The potassium ion efflux channel GORK plays a critical role in closing plant leaf stomata by releasing K+ from guard cells to reduce guard cell volume and turgor. The GUARD CELL OUTWARD-RECTIFYING K+ (GORK) channel is expressed in Arabidopsis guard cells and encodes a K+out channel. Voltage-dependent K+ channels, including GORK, contain three regions: an intracellular N-terminal region, a transmembrane region, and an intracellular C-terminal region (27–30). The transmembrane region is composed of six transmembrane helices (S1-S6), with S1-S4 forming the voltage sensing domain and S5 and S6 forming the pore region.

As a result, five different structures of GORK ranging from the transmembrane region to the C-terminal ANK (designated as GORKWT1–GORKWT5) were determined at resolutions of 3.16 to 3.27 Å. The five GORK structures showed N-terminally an almost uniform transmembrane domain (positions 50 to 313 from the initial Met), including the voltage-sensing domain and the ion selectivity filter. In contrast, the following cytosolic regions, i.e., C-linker (positions 314 to 364), CNBD (positions 365 to 490), CNBD–Ankyrin bridge (positions 491 to 542), and ANK (positions 543 to 722) show five distinct structures in almost twofold symmetry (C2 symmetry). Furthermore, overlaying GORKWT1 and GORKWT5, which had high resolutions of 3.17 and 3.16 Å, respectively, revealed that one of the C-linkers in each dimer was pushed upward by the CNBD in GORKWT1, as compared to GORKWT5. Closer inspection of the structure revealed that the difference of the degree of bending in the C-linker between Mol I and Mol II was small in GORKWT1 but greater in GORKWT5. Additionally, GORKWT1 displayed a C4-like C2 symmetry in the CNBD, whereas GORKWT5 showed a pronounced C2 symmetry. Furthermore, we found a structural difference in the short structure that lies between the CNBD and ANK domains, termed as CNBD–Ankyrin bridge containing residues 511 to 519. This region had an α-helical structure in GORKWT1, while in GORKWT5, it was entirely present in a nonhelical loop conformation. The Cryo-EM structural data showed that K514 likely formed salt bridges with E508, E517, and D511 in GORKWT1, and that L516 engaged in hydrophobic interaction with I457, P466, and F467 in GORKWT1. Thus, the rigidity provided by the α-helix in the CNBD–Ankyrin bridge apparently contributed to the stability toward a C4 symmetry in the C-linker and the CNBD.

>[4x]MDYKDDDDKGRLRRRQEIIDHEEEESNDDVSSRRGKLSLAETFRWLDSSEHRRIETDGHNDYKYIIHPKNRWYKAWEMFILVWAIYSSLFTPMEFGFFRGLPERLFVLDIVGQIAFLVDIVLQFFVAYRDTQTYRTVYKPTRIAFRYLKSHFLMDFIGCFPWDLIYKASGKHELVRYLLWIRLFRVRKVVEFFQRLEKDTRINYLFTRILKLLFVEVYCTHTAACIFYYLATTLPPENEGYTWIGSLKLGDYSYENFREIDLWKRYTTALYFAIVTMATVGYGDIHAVNLREMIFVMIYVSFDMVLGAYLIGNITALIVKGSNTERFRDKMNDLISFMNRKKLGRDLRSQITGHVRLQYDSHYTDTVMLQDIPASIRAKIAQLLYLPYIKKVPLFKGCSTEFINQIVIRLHEEYFLPGEVITEQGNVVDHLYFVCEGLLEALVTKTDGSEESVTLLGPHTSFGDISIICNISQPFTVRVCELCHLLRLDKQSFSNILEIYFHDGRTILNNIMEEKESNDRIKKLESDIVIHIGKQEAELALKVNSAAFQGDFYQLKSLIRSGADPNKTDYDGRSPLHLAACRGYEDITLFLIQEGVDVNLKDKFGHTPLFEAVKAGQEGVIGLLVKEGASFNLEDSGNFLCTTVAKGDSDFLKRLLSSGMNPNSEDYDHRTPLHVAASEGLFLMAKMLVEAGASVISKDRWGNSPLDEARLCGNKKLIKLLEDVKNAQSSIYPSSLRELQEERIERRKCTVFPFHPQEAKEERSRKHGVVVWIPSNLEKLIVTAAKELGLSDGASFVLLSEDQGRITDIDMISDGHKLYMISDTTDQTHHHHHH>[8x]MAGKAHRLSAEERDQLLPNLRAVGWNEL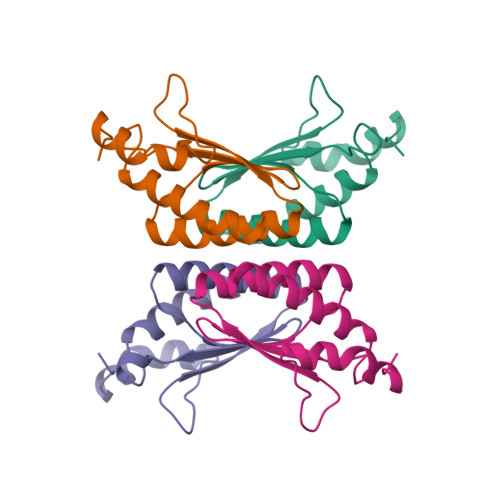EGRDAIFKQFHFKDFNRAFGFMTRVALQAEKLDHHPEWFNVYNKVHITLSTHECAGLSERDINLASFIEQVAVSMT> MKPKVFITREIPEVGIKMLEDEFEVEVWGDEKEIPREILLKKVKEVDALVTMLSERIDKEVFENAPKLRIVANYAVGYDNIDIEEATKRGIYVTNTPDVLTDATADLAFALLLATARHVVKGDRFVRSGEWKKRGVAWHPKWFLGYDVYGKTIGIIGLGRIGQ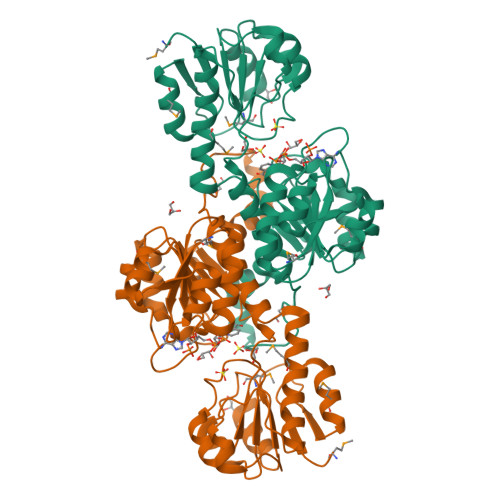AIAKRAKGFNMRILYYSRTRKEEVERELNAEFKPLEDLLRESDFVVLAVPLTRETYHLINEERLKLMKKTAILINIARGKVVDTNALVKALKEGWIAGAGLDVFEEEPYYNEELFKLDNVVLTPHIGSASFGAREGMAELVAKNLIAFKRGEIPPTLVNREVIKIRKPGFE Recently, the ykkC RNA motif was identified as binding to multiple, chemically dissimilar ligands, which makes this specific scaffold a compelling target for structural studies of RNA evolvability (Sherlock et al., 2018a; 2018b; Nelson et al., 2017). Subtype 2b is responsive to phosphoribosyl pyrophosphate (PRPP), a precursor in purine biosynthesis. To address these questions of molecular recognition by RNA, we report the near-atomic resolution structure of a native ykkC 2b riboswitch in complex with PRPP via X-ray crystallography. We also convert this construct into a ppGpp aptamer with a single G96A mutation and present the structure of the mutant bound to ppGpp.

To understand the basis of ligand recognition by the PRPP riboswitch, we determined the crystal structure of the aptamer domain of the ykkC 2b riboswitch from Thermoanaerobacter mathranii at 2.5 Å resolution in the presence of its native ligand, PRPP. Like its parent aptamer, the PRPP riboswitch contains two adjacent helical stacks. However, unlike the guanidine aptamer, the PRPP aptamer has structured tails at the 5′ and 3′ ends that are not conserved in the guanidine riboswitch. The ends pair to form an additional short helix that we have termed P0, resulting in a four-way junction between P0, P1, P2, and P3. P0 coaxially stacks with P3 and extends the binding pocket for recognition of the larger PRPP ligand. One metal (M1) associates with the 5-phosphate, and the second metal (M2) associates with the pyrophosphate. Both metals form contacts bridging PRPP and the RNA aptamer. Equivalent to G89 in guanidine-I, G96 flips out and base pairs with C75 while also hydrogen bonding to PRPP. The present results show that the PRPP aptamer recognizes its ligand through a shifted and extended helical ligand-binding region, allowing for the retention of bound metal ions and extensive hydrogen bond donation to phosphate groups. The wild-type aptamer shows low affinity for ppGpp (Kd = 91 ± 3 μM) and 46-fold greater affinity for PRPP (Kd = 2.0 ± 0.3 μM).

>GUGAAAGUGUACCUAGGGUUCCAGCCUAUUUGUAGGUGUUCGGACCGAGCGGUACAGGUAUAUUUUUAUAUACCACACCUUAGGGACAAAAGCCCGGGAGGAUAGGUUUCACUCGUA[2x]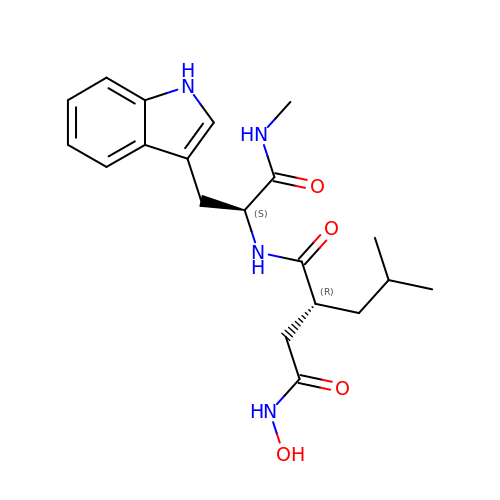3-(N-HYDROXYCARBOXAMIDO)-2-ISOBUTYLPROPANOYL-TRP-METHYLAMIDE | C20 H28 N4 O4 | NITYDPDXAAFEIT-DYVFJYSZSA-N1-BROMOETHANE | C2 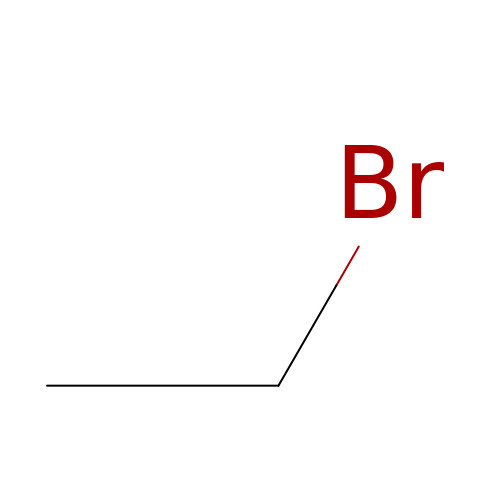H5 Br | RDHPKYGYEGBMSE-UHFFFAOYSA-N>[3x]MAEKTFKVV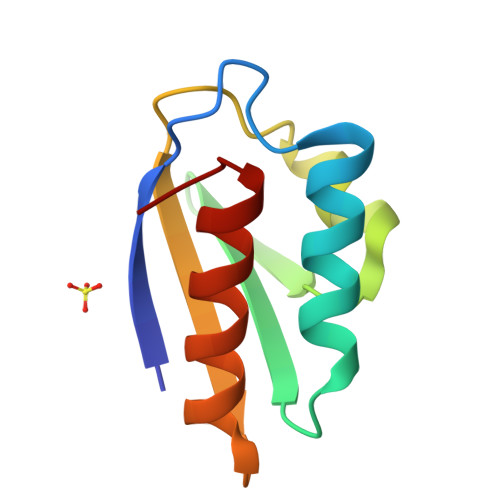SDSGIHARPATILVQTASKFNSEIQLEYNGKTVNLKSIMGVMSLGIPKGATIKITAEGADAAEAMAALTDTLAKEGLAE>[2x]MVLYFIGLGLYDERDITVKGLEIAKKCDYV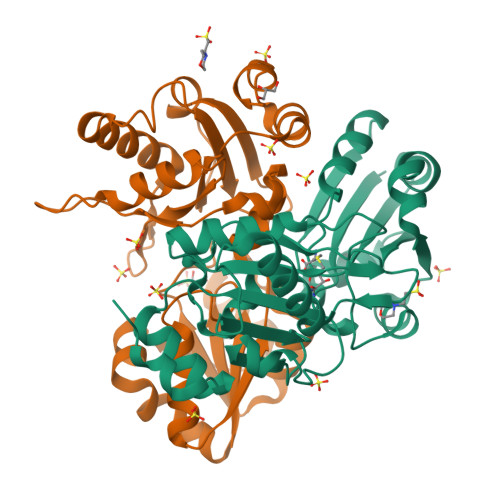FAEFYTSLMAGTTLGRIQKLIGKEIRVLSREDVELNFENIVLPLAKENDVAFLTPGDPLVATTHAELRIRAKRAGVESYVIHAPSIYSAVGITGLHIYKFGKSATVAYPEGNWFPTSYYDVIKENAERGLHTLLFLDIKAKKRMYMTANEAMELLLKVEDMKKGGVFTDDTLVVVLARAGSLNPTIRAGYVKDLIREDFGDPPHILIVPGKLHIVEAEYLVEIAGAPREILRVNV>MLTSLIHSKETINKTQTSTAADSAMEYILFYISKAIAQAKRLTYAQFFDSTGRLIYTGDSFENDYLNTFNSYIADFFENRGNRIGIDMKLADNSSVQVSNVSELILLARQSCEYISNISFSRSGNSYILEVEALDSTTKTKRVERCVFTIPSPFEKVEIVSNSSSPDTLLPYLLAWDSNIFDFTTYGLFSSDKIIFNNNITVTTRNMYSSSDITLRSDNNRPGDYTIKADNIIVKNGSFIFGGNNKVVVNNLMYTKNGITFNGNNNRLESNSLLFSDGTISLSGKDEIVANALFCDTLDIRNGSSNLVTINEFAYFNKL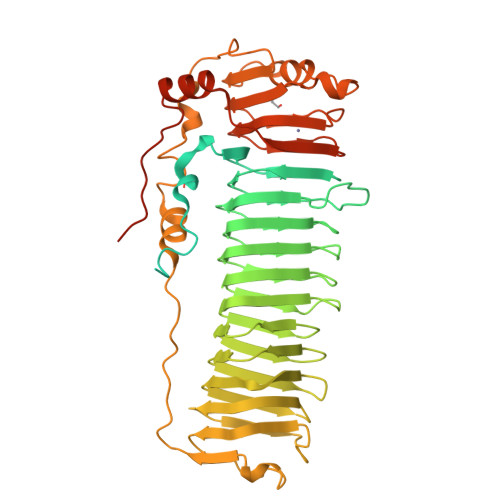NIWTDKMVLKSNSKLFGGDIEIRNDGILSADVGTVVYANNLDIIGSSATIDAPDTVLYCNNLKIDGEVKLNVKKIVCSGTITISNLNSGTNIRVSDKIECRSIPQNIPSGIRNLFVQNPNVNFQIPYPTIPAIIEEIKKNTFPTNWIRLDNIVEDKKDINGANYYSLVSTGQNSNDINEIFNKNKPNNPHSNVQIFVITKSGINVPPDQNHLDGVLIANGSLQFNGGNLNIEYVRMPQPLIDYLLSKNIIKIENVQPPVISNPTVTFLPRDVNLFIIARHFVVK[2x]>[6x]MTGNDVQGAEKADAIGMVLGTEDVTPTVFWFAVSH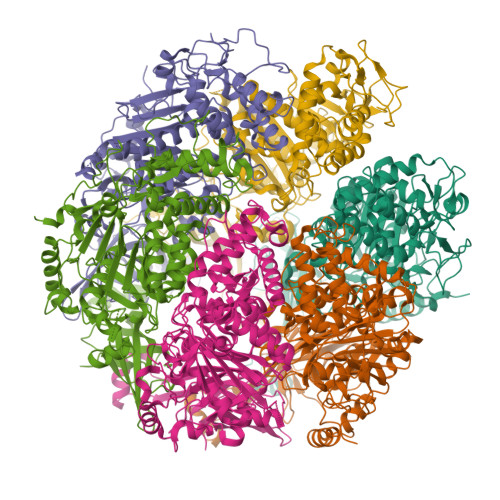GASVGLDDLVVVETRKPDGTPVRFYGLVDNVRKRHEGVTFESDVEDVVAGLLPASVSYAARVLVTRVDPENFIPPQPGDHVRHAAGRELAMALSADKMEEAAFPGGLLADGQPLPLNFRFINGESGGHINISGISGVATKTSYALFLLHSIFRSGVMDRTAQGSGGRQSGTAGGRALIFNVKGEDLLFLDKPNARMVEKEDKVVRAKGLSADRYALLGLPAEPFRDVQLLAPPRAGAAGTAIVPQTDQRSEGVTPFVFTIREFCARRMLPYVFSDASASLNLGFVIGNIEEKLFRLAAAQTGKGTGLIVHDWQFEDSETPPENLDFSELGGVNLQTFEQLISYLEYKLLEEREGEGDPKWVLKQSPGTLRAFTRRLRGVQKYLSPLIRGDLTPEQAEGYRPDPLRRGIQLTVVDIHALSAHAQMFVVGVLLREVFEYKERVGRQDTVFVVLDELNKYAPREGDSPIKDVLLDIAERGRSLGIILIGAQQTASEVERRIVSNAAIRVVGRLDLAEAERPEYRFLPQSFRGRAGILQPGTMLVSQPDVPNPVLVNYPFPAWATRRDEVDDLGGKAAAEVGAGLLR>[12x]MPGSIPLIGERFPEMEVTTDHGVIKLPDHYVSQGKWFVLFSHPADFTPVSTTEFVSFARRYEDFQRLGVDLIGLSVDSVFSHIAWKEWIERHIGVRIPFPIIADPQGTVARRLGLLHAESATHTVRGVFIVDARGVIRTMLYYPMELGRLVDEILRIVKALKLGDS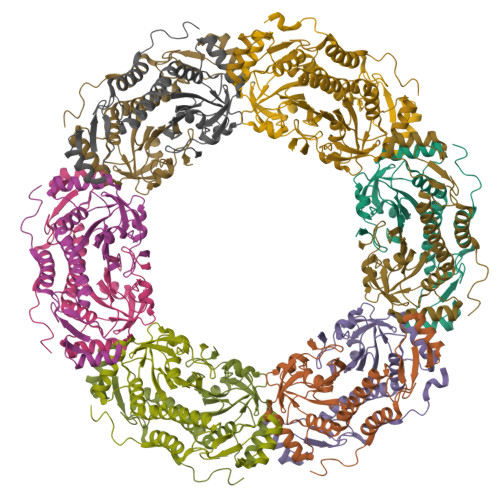LKRAVPADWPNNEIIGEGLIVPPPTTEDQARARMESGQYRSLDWWFSWDTPASRDDVEEARRYLRRAAEKPAKLLYEEARTHLH> MCSAGGIRRPIQIEEFKTAISGMSDMELAQIKTEIENSINHLQRSN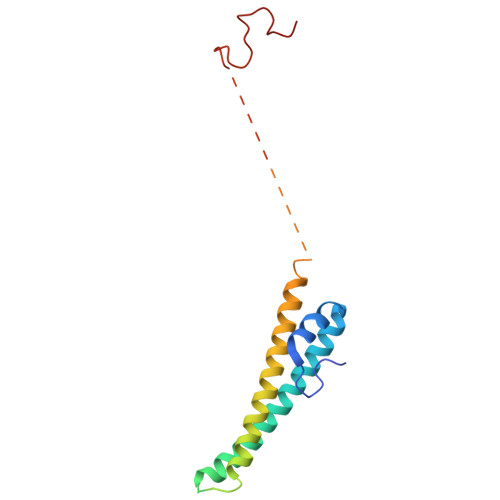ARLGKYIAKLEGADDRLEADDSDDLENIDSGDLALYKDSVRENEIVLNNYNERVDALEQETVYRKTGHGKSKHEVEAKDNTNKGPDVDMDNSNVDVVTPNSIFI OCTANOIC ACID [3S-[3ALPHA, 3ABETA, 4ALPHA, 6BETA, 6ABETA, 7BETA, 8ALPHA(Z), 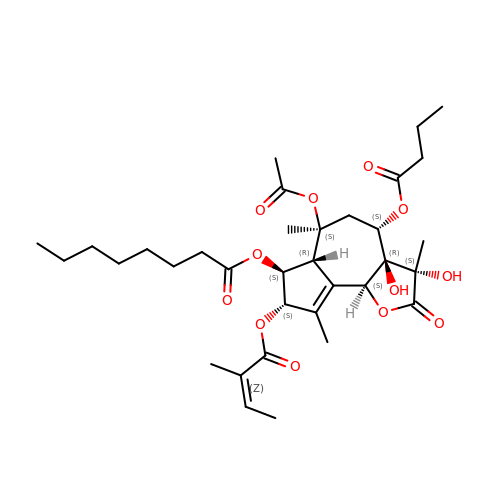9BALPHA]]-6-(ACETYLOXY)-2,3,-3A,4,5,6,6A,7,8,9B-DECAHYDRO-3,3A-DIHYDROXY-3,6,9-TRIMETHYL-8-[(2-METHYL-1-OXO-2-BUTENYL)OXY]-2-OXO-4-(1-OXOBUTOXY)-AZULENO[4,5-B]FURAN-7-YL ESTER | C34 H50 O12 | IXFPJGBNCFXKPI-FSIHEZPISA-N IMPDH catalyzes the NAD+-dependent conversion of inosine 5’-monophosphate (IMP) to xanthosine 5’-monophosphate (XMP), the first of the two step biosynthesis of guanosine 5’-monophosphate (GMP). Inosine 5’-monophosphate dehydrogenase (IMPDH) lies at a key intersection of the purine biosynthesis pathway and represents an extremely attractive target since it controls flux of the guanine nucleotide pool. We have overcome this major limitation by designing a variant that lacks the non-catalytic CBS subdomain (MtbIMPDH2ΔCBS), greatly improving solubility without impacting enzyme catalytic properties. Here we present the first crystal structures of MtbIMPDH2ΔCBS, including the apoenzyme, the E•XMP•NAD+ complex, and complexes with IMP and three inhibitors, MAD1, P41, and Q67.

The structure of the tertiary complex of MtbIMPDH2ΔCBS with XMP and NAD+ was obtained by soaking crystals containing the MtbIMPDH2ΔCBS•IMP complex with 200 mM NAD+. The 1.60 Å resolution crystal structure of the product/cofactor complex contains one protein chain per asymmetric unit. Although no potassium was present in the crystallization buffer and this ion is not found in the complex, the high quality electron density maps clearly show that the product XMP is present in the active site. This indicates that the enzyme in the crystal is catalytically competent. As observed for VcIMPDHΔCBS•XMP•NAD+, the NAD+ adenosine moiety binds in the AB-subsite located at the subunit interface and interacts with residues from both monomers. However, the nicotinamide ring flips ~180° and is in a syn-conformation in MtbIMPDH2ΔCBS•XMP•NAD+ (with χN torsion angle of 5.7°). The carboxamide moiety makes direct hydrogen bonds with side chains of T343, E458, and Y487’ (which is a part of the IMSM) and a water-mediated interaction with the O1N atom of the phosphate group and the N7A atom of adenine. As a result of the syn-conformation, the pro-R side of the nicotinamide ring now faces IMP with its C4N carbon aligned with the C2 of the IMP hypoxanthine ring (C4N-C2 distance of 3.28 Å). The deuterium also transferred to the pro-S position of NAD+ in the MtbIMPDH2ΔCBS catalyzed reaction. These observations indicate that the orientation of NAD+ observed in the XMP complex is not competent for hydride transfer and may reflect cofactor conformation stabilized by the IMSM.

> SNAMSRGMSGLEDSSDLVVSPYVRMGGLTTDPVPTGGDDPHKVAMLGLTFDDVLLLPAASDVVPATADTSSQLTKKIRLKVPLVSSAMDTVTESRMAIAMARAGGMGVLHRNLPVAEQAGQVEMVKRSGGLLVGAAVGVGGDAWVRAMMLVDAGVDVLVVDTAHAHNRLVLDMVGKLKSEVGDRVEVVGGNVATRSAAAALVDAGADAVKVGVGPGSICTTRVVAGVGAPQITAILEAVAACRPAGVPVIADGGLQYSGDIAKALAAGASTAMLGSLLAGTAEAPGELIFVNGKQYKSYRGMGSLGAMRGRGGATSYSKDRYFADDALSEDKLVPEGIEGRVPFRGPLSSVIHQLTGGLRAAMGYTGSPTIEVLQQAQFVRITPAGLKESHPHDVAMTVEAPNYYAR> ATRELDELMASLSDF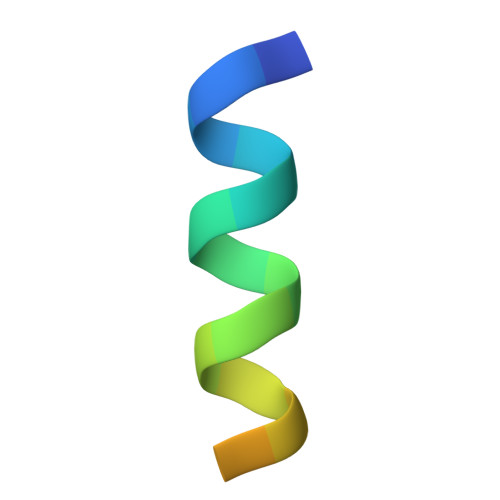KFMAQ> MIEVKPINAEDTYELRHRILRPNQPIEACMFESDLLRGAFHLGGYYGGKLISIASFHQAEHSELQGQKQYQLRGMATLEGYREQKAGSSLIKHAEEILRKRGADLLWCNARTSASGYYKKL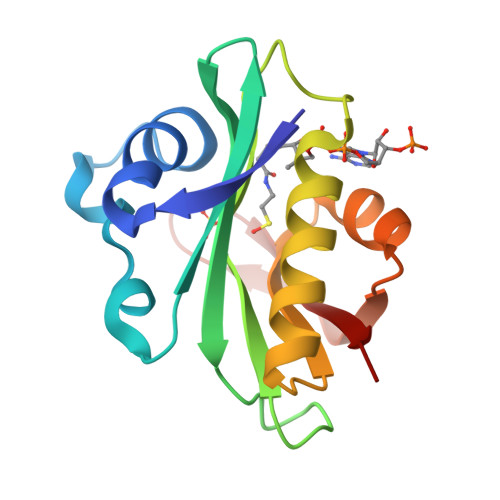GFSEQGEVFDTPPVGPHILMYKRIT> MSIMLPINNNFSLSQNSFYNTISGTYADYFSAWDKWEKQALPGENRNEAVSLLKECLINQFSELQLNRLNLSSLPDNLPPQITVLEITQNALISLPELPASLEYLDACDNRLSTLPELPASLKHLDVDNNQLTMLPELPALLEYINADNNQLTMLPELPTSLEVLSVRNNQLTFLPELPESLEALDVSTNLLESLPAVPVRNHHSEETEIFFRCRENRITHIPENILSLDPTCTIILEDNPLSSRIRESLSQQTAQPDYHGPRIYFSMSDGQQNTLHRPLADAVT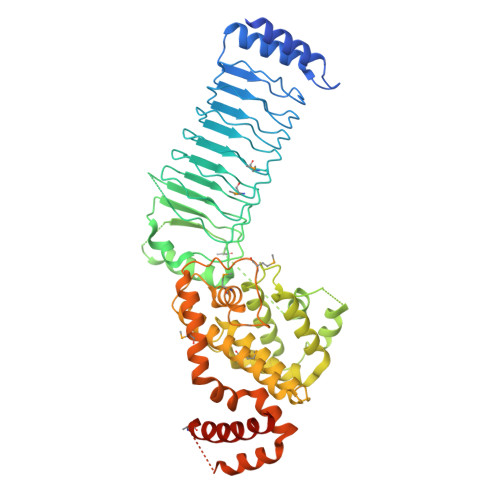AWFPENKQSDVSQIWHAFEHEEHANTFSAFLDRLSDTVSARNTSGFREQVAAWLEKLSASAELRQQSFAVAADATESCEDRVALTWNNLRKTLLVHQASEGLFDNDTGALLSLGREMFRLEILEDIARDKVRTLHFVDEIEVYLAFQTMLAEKLQLSTAVKEMRFYGVSGVTANDLRTAEAMVRSREENEFTDWFSLWGPWHAVLKRTEADRWALAEEQKYEMLENEYPQRVADRLKASGLSGDADAEREAGAQVMRETEQQIYRQLTDEVLALRLPENGSQLHHS>[8x]AGGKVTSSTGIAPKRYVYYPGSEELGPD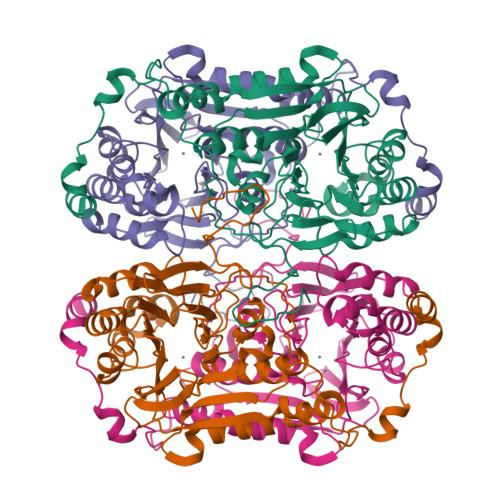EIRVIACGTGMPTARRAQAAAAWVVELGNGDKFIVDIGSGSMANIQSLMIPANYLTKIFLTHLHTDHWGDLVSMWAGGWTAGRTDPLEVWGPSGSREDMGTKYAVEHMLKAYNWDYMTRAVTINPRPGDINVHEFDYRALNEVVYQENGVTFRSWPCIHAGDGPVSFALEWNGYKVVFGGDTAPNIWYPEYAKGADLAIHECWMTSDQMMTKYNQPAQLALRINLDFHTSAQSFGQIMNMVQPRHAVAYHFFNDDDTRYDIYTGVRENYAGPLSMATDMMVWNITRDAVTERMAVSPDHAWDVAGPSEDLAPDRNRASEYTQYILDGRLNVDEANAHWKQEFMG> MSAQVMLEDMARKYAILAVKADKEGKVEDAITYYKKAIEVLSQIIVLYPESVARTAYEQMINEYKKRISYLEKVLPASSDGSG;> MSAQVMLEDMARKYAILAVKADKEGKVDD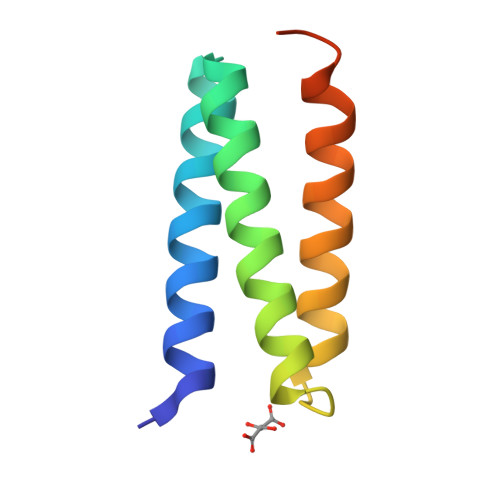AITYYKKAIEVLSQIIVLYPESVARTAYEQMINEYKKRISYLEKVLPASSDGSG> VSITKCSSDMNGYCLHGQCIYLVDMSQNYCRCEVGYTGVRCEHFFLT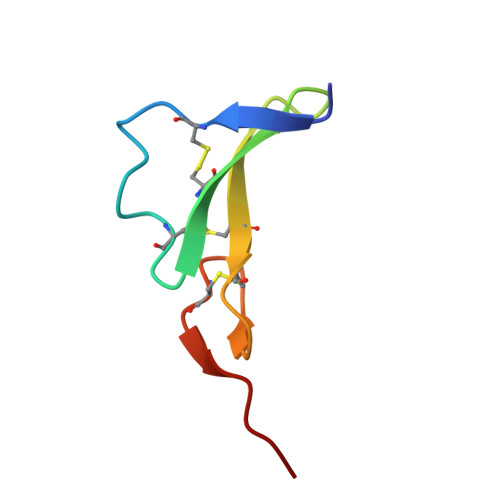V6-{2-[(2,4-diamino-5-methylpyrido[2,3-d]pyrimidin-6-yl)methyl]-4-methoxyphenyl}hex-5-ynoic acid | C22 H23 N5 O3 | 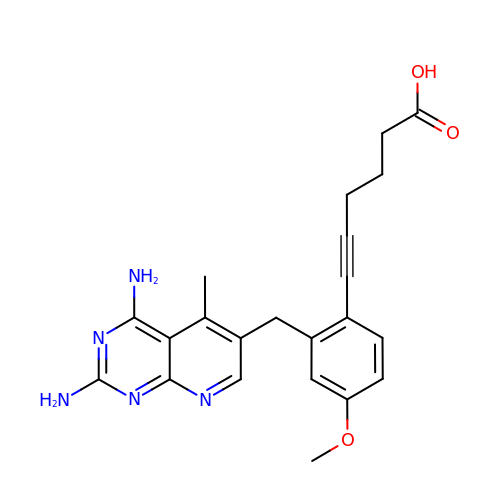MAWHZPJVFGJFTF-UHFFFAOYSA-N> SRTGYDNREIVMKYIHYKLSQRGYEWDAGDDVEENRTEAPEGTESEVVHLTLRQAVDDFSRRYRRDFAEMSSQLHLTPFTARGRFATVVEELFRDGVNWGRIVAFFEFGGVMCVESVNREMSPLVD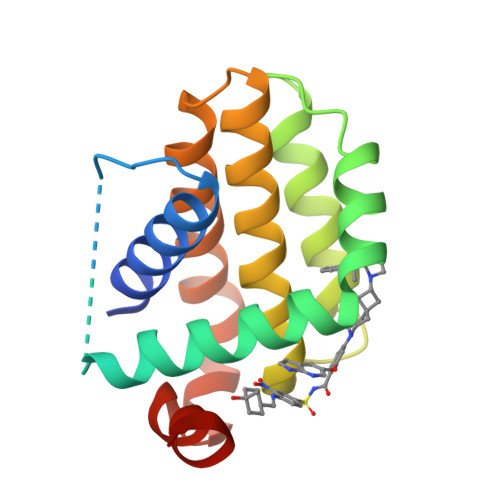NIALWMTEYLNRHLHTWIQDNGGWDAFVELYGPSMR> SVSIGYLLVKHSQTDQEPMCPVGMNKLWSGYSLLYFEGQEKAHNQDLGLA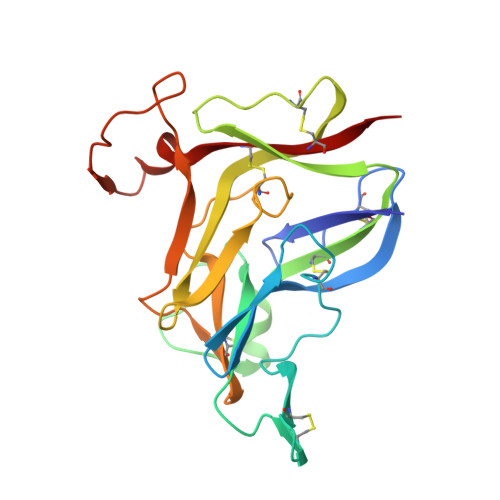GSCLARFSTMPFLYCNPGDVCYYASRNDKSYWLSTTAPLPMMPVAEDEIKPYISRCSVCEAPAIAIAVHSQDVSIPHCPAGWRSLWIGYSFLMHTAAGDEGGGQSLVSPGSCLEDFRATPFIECNGGRGTCHYYANKYSFWLTTIPEQSFQGSPSADTLKAGLIRTHISRCQVCMKNL> MFYSLMRESKIVIEYDGRGYHFDALSNYDASTSFQEFKTLRRTIHNRTNYADSIINAQDPSSISLAINFSTTLIESNF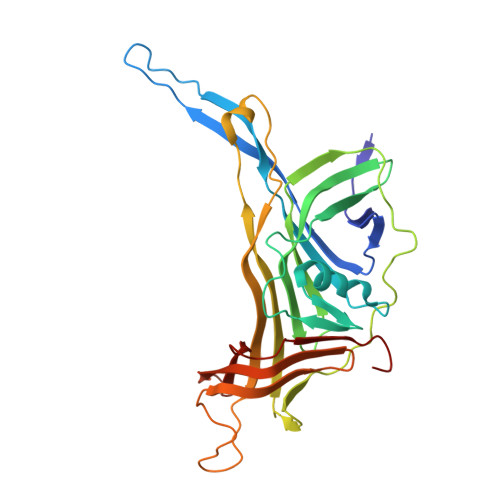FDWMGFTREGNSLFLPRNTPNIEPIMFNMYIINHNNSCIYFENCYVSTVDFSLDKSIPILNVGIESGKFSEVSTFRDGYTITQGEVLPYSAPAVYTNSSPLPALISASMSFQQQCSWREDRNIFDINKIYTNKRAYVNEMNASATLAFYYVKRLVGDKFLNLDPETRTPLIIKNKYVSITFPLARISKRLNFSDLYQVEYDVIPTADSDPVEINFFGERK>MTTNLTNSNCVEEYKENGKTKIRIKPFNALIELYHHQTPTGSIKENLDKLENYVKDVVKAKGLAIPTSGAFSNTRGTWFEVMIAIQSWNYRVKRELNDYLIIKMPNVKTFDFRKIFDNETREKLHQLEKSLLTHKQQVRLITSNPDLLIIRQKDLIKSEYNLPINKLTHENIDVALTLFKDIEGKCKWDSLVAGVGLKTSLRPDRRLQLVHEGNILKSLFAHLKMA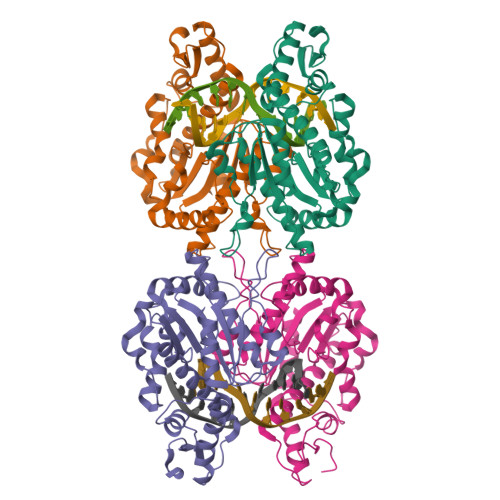YWNPKAEFKYYGASSEPVSKADDDALQTAATHTIVNVNSTPERAVDDIFSLTSFEDIDKMLDQIIKK[8x]> MGIGIYSPGIWRIPHLEKFLAQPCQKLSLLRPVPQEVNAIAVWGHRPSAAKPVAIAKAAGKPVIRLEDGFVRSLDLGVNGEPPLSLVVDDCGIYYDASKPSALEKLVQDKAGNTALISQAREAMHTIVTGDMSKYNLAPAFVADESERTNIVLVVDQTFNDMSVTYGNAGPHEFAAMLEAAMAENPQAEIWVKVHPDVLEGKKTGYFADLRATQRVRLIAENVSPQSLLR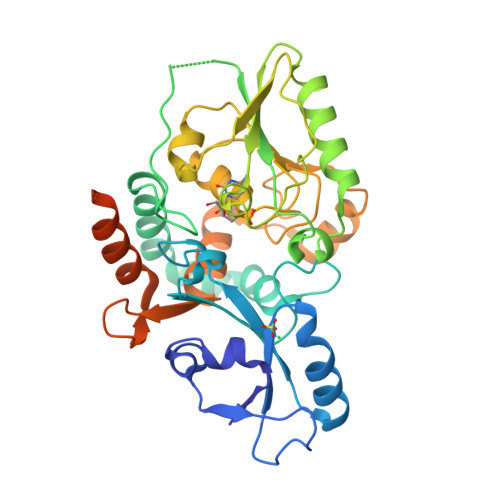HVSRVYVVTSQYGFEALLAGKPVTCFGQPWYASWGLTDDRHPQSALLSARRGSATLEELFAAAYLRYCRYIDPQTGEVSDLFTVLQWLQLQRRHLQQRNGYLWAPGLTLWKSAILKPFLRTPTLEHHHHHH>[4x]MRGSHHHHHHGSMKRAVITGLGIVSSIGNNQQEVLASLREGRSGITFSQELKDSGMRSHVWGNVKLDTTGLIDRKVVRFMSDASIYAFLSMEQAIADAGLSPEAYQNNPRVGLIA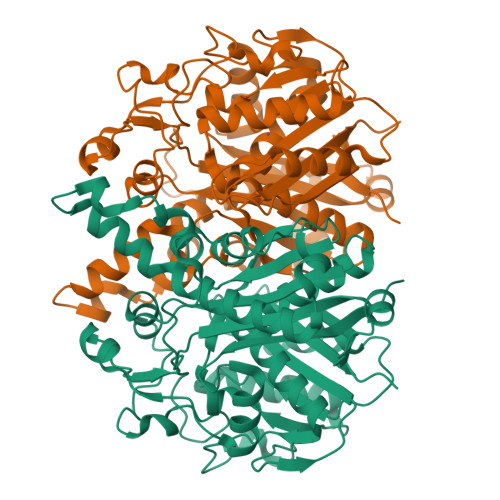GSGGGSPRFQVFGADAMRGPRGLKAVGPYVVTKAMASGVSACLATPFKIHGVNYSISSACATSAHCIGNAVEQIQLGKQDIVFAGGGEELCWEMACEFDAMGALSTKYNDTPEKASRTYDAHRDGFVIAGGGGMVVVEELEHALARGAHIYAEIVGYGATSDGADMVAPSGEGAVRCMKMAMHGVDTPIDYLNSQGTSTPVGDVKELAAIREVFGDKSPAISATKAMTGHSLGAAGVQEAIYSLLMLEHGFIAPSINIEELDEQAAGLNIVTETTDRELTTVMSNSFGFGGTNATLVMRKLKD>NYPAEPFRIKSVETVSMIPRDERLKKMQEAGYNTFLLNSKDIYIDLLTDSGTNAMSDKQWAGMMMGDEAYAGSENFYHLERTVQELFGFKHIVPTHQGRGAENLLSQLAIKPGQYVAGNMYFTTTRYHQEKNGAVFVDIVRDEAHDAGLNIAFKGDIDLKKLQKLIDEKGAENIAYICLAVTVNLAGGQPVSMANMRAVRELTAAHGIKVFYDATRCVENAYFIKEQEQGFENKSIAEIVHEMFSYADGCTMSGKKDCLVNIGGFLCMNDDEMFSSAKELVVVYEGMPSYGGLAGRDMEAMAIGLREAMQYEYIEHRVKQVRYLGDKLKAAGVPIVEPVGGHAVFLDARRFCEHLTQDEFPAQSLAASIYVETGVRSMERGIISAGRNNVTGEHHRPKLETVRLTIPRRVYTYAHMDVVADGIIKLYQHKEDIRGLKFI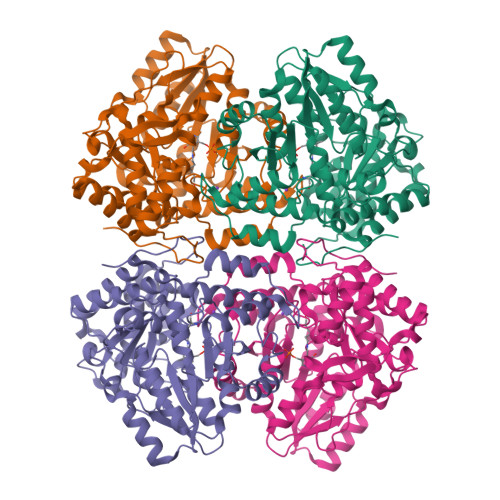YEPKQLRAFTARFDYI[2x]> MFGRTAFLLRKYRQKSKAPDLKTSFSKTRNFKKAEKIAIETVDGEVVKGRGKLRRRSHSALKKAIGEMEHPSIWLWYPWRMNPEPPTPGMPQRRALKNLHGAVFTDLTPVQKKRQEQMLYGINIPETRQMKFEQEHPLLASALRQLDGQPKGFPFWYKKYPTRRHAYGNRFSIPDEMLEGYGEEMKKALSKEMMSIQEKQFAQEAMYMERYAEHDFDTTSPAVLAVKRALKCRVLRNHLLTNPHNNIIKAVLANTE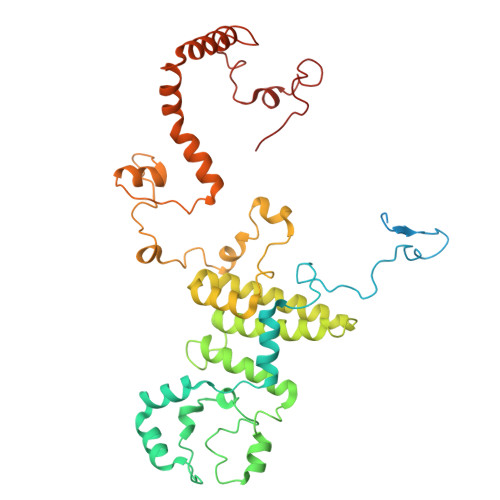KKLSHALRKLRKVDFKKYWEIIRDHDVQDVLQPSNLVTYRQGAYWKYDWNAGLAISTNLADVLDPRGLNGCVETGRSRSEVARDLGLSYTRPLQENEKKQLSHQALYYERLAKFKMEQPEAARALERERFVRKFSGMFAKMDIKSGAPDFPSTYRKLLGTKVVRWASKRHGPA> MAPTNPLTLIVATTPIPTREKTLLGIGLNGTLPWPRIKADMSFFARVTTRPPRPGTTNAMIMGRKTYDSVPKSLRPLGKRINVIVTRDVEGVSKRVAE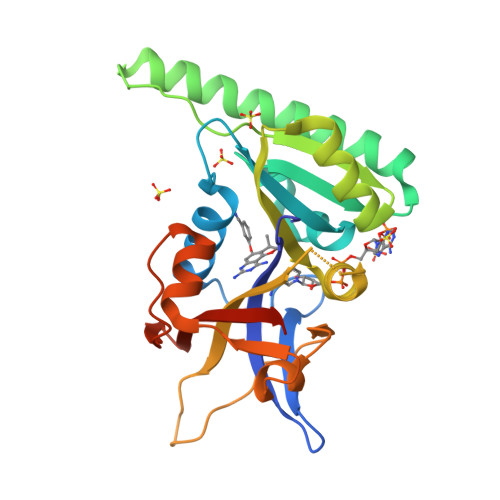ELKEKRAKMAAAAAAATSAGENKEEGPITDAIVSSGLEAALEDVEEKFKGGLGSVFVIGGAEIYATALGLGGDRPVRIVMTNVEKKGVDGEKAVFECDTFFPIDEELLMEKGWRKVSAEEVTEWVGEPVSGEWKDEGEVRIQMVGYERVNLEHHHHHH> GMEPSAKHLQLQTLLSERHAYLMEGNREAMHQLLSSDFSFIDGQGRQFDAETYLDHYVDPDQIQWSNQISESMVVEVFETTALVQEIVEDHFSYGRSMYIGRFRSVSLYHWANEGWKWHFHQLT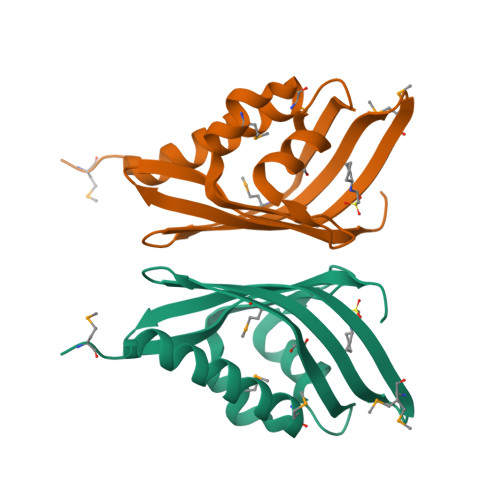PLDPS> MGSSHHHHHHLTISIDIKAEDRKYQIVENSVTSILFKVSDTTTRYVYNIRMGEMRNESETTPEGLKNLNLKKECDLSVKIRTEADQAFVLSEKHRGNIMLVEFFKYEGIPVLCASCVLIVKPSDLKITQVIFKDSTGKEVGCGSVQYEANLKFALRVKYNRPLLRGEKAPKLKCKGYCTNAVTGEYEEISKFRVDENGAYTDTFYCDDGLQESHAGADYVFSFGINNPYGPPFMIEDTNVPVPSIQKIHLIGRNLKKPQITSV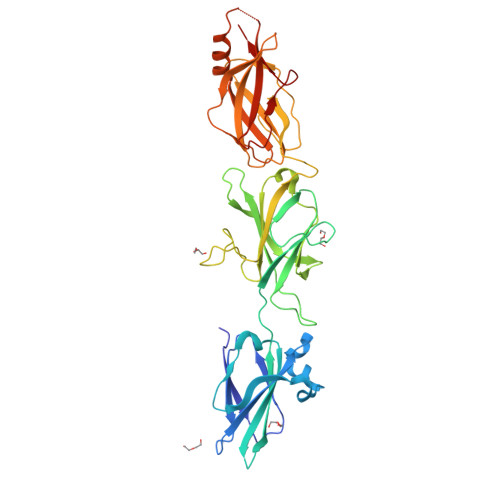IWSSKEMIKFGEDSPRRKSINYNEDGFLHIHARGMYGQKVRVELFEKDSTGIKKLLLGLKDDVTILDNVVCVPVEMSGVYAKAAKGRHALAEGLSFEILAKVTPLDTSIAAFEQDDKSLIELQIYGK>[4x]MASLQLLPSPTPNLEIKYTKIFINNEWQNSESGRVFPVCNPATGEQVCEVQEADKVDIDKAVQAARLAFSLGSVWRRMDASERGRLLDKLADLVERDRATLATMESLNGGKPF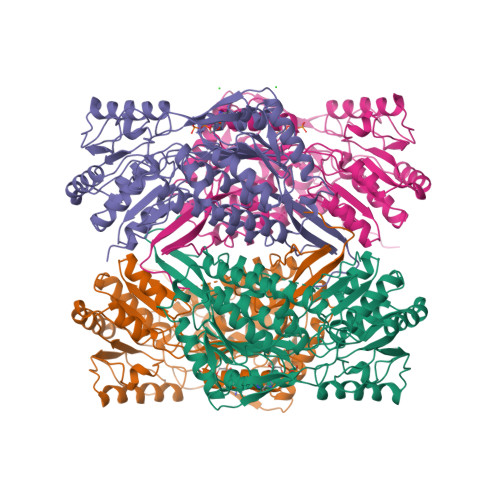LQAFYIDLQGVIKTLRYYAGWADKIHGMTIPVDGDYFTFTRHEPIGVCGQIIPWNFPLLMFTWKIAPALCCGNTVVIKPAEQTPLSALYMGALIKEAGFPPGVVNILPGYGPTAGAAIASHIGIDKIAFTGSTEVGKLIQEAAGRSNLKRVTLELGGKSPNIIFADADLDYAVEQAHQGVFFNQGQCCTAGSRIFVEESIYEEFVKRSVERAKRRIVGSPFDPTTEQGPQIDKKQYNKILELIQSGVAEGAKLECGGKGLGRKGFFIEPTVFSNVTDDMRIAKEEIFGPVQEILRFKTMDEVIERANNSDFGLVAAVFTNDINKALMVSSAMQAGTVWINCYNALNAQSPFGGFKMSGNGREMGEFGLREYSEVKTVTVKIPQKNS>MVAPITTSGNKVLFGGQQGSIAGNSFFWSNTGWGGEKYYNAQTVAWLKSDWKSSLVRAAMGVDESGGYITDSYNKTRVTTVVDAAIANNMYVIIDWHSHHAEQYQSQAIAFFKEMATKYGNNNNVIYEIYNEPLQVSWSSVIKPYATAVIAEIRKIDPDNLIVVGTPTWSQDVDVAANDPITGYANIAYTLHFYAGTHGQSLRNKASTALSKGIPLFVTEWGSVNADGGGSVATAETNSWVSFMKTNNISNANWALNDKAEGASALVSGASANGGWTSSQLTASGTLAKSIISGWP[2x]

Here, we report a novel cellulase belonging to GH5 family, named as CelE1, retrieved from a sugarcane soil metagenomic library, which is a promising biocatalyst in biofuels production. CelE1 is 1284 bp long and encodes a polypeptide of 428 amino acid residues containing a putative N-terminal signal peptide followed by a glycoside hydrolase domain belonging to family 5 (GH5). Cellulases or endoglucanases (EC 3.2.1.4) catalyze the cleavage of random internal β-1,4-glycosidic bonds in cellulosic chains and can be found coupled to the cellulosome or generally secreted as independent enzymes. A new plant cell wall-degrading enzyme with ability to breakdown complex cellulose-based substrates was isolated and characterized from sugarcane soil metagenome. This enzyme was shown to be an endo-acting glucanase with high catalytic activity at a broad temperature range and under alkaline conditions that usually cause enzyme inactivation of classical acidic cellulases.

The structure of this novel cellulase 5 was determined by X-ray crystallography at 1.8 Å resolution. The crystals belonged to the monoclinic space group P21 with two molecules in the asymmetric unit, which could suggest a quaternary arrangement. However, analysis of crystalline contacts using the PDBePISA server did not indicate the presence of any stable protein–protein interface discarding the existence of CelE1 as a dimer in solution. The enzyme displays a canonical (β/α)8-barrel fold (also known as TIM-barrel) characteristic for members of GH5 family, which is composed by eight β-sheets surrounded by eight α-helices. The long loops connecting the C-terminal end of β-strands with the N-termini of the external layer of helices delineate the negatively charged catalytic cleft. By comparison with other cellulases the residues Glu152 and Glu240 were identified as the catalytic acidic residues, where Glu152 is the proton donor and Glu240 the nucleophile. These residues are separated by a distance of 6.1 Å, compatible for a retaining catalytic mechanism. Other important residues for catalysis are conserved including His117 and His212 and the aromatic gatekeepers Trp189 and Trp241. Despite the fully conserved catalytic cleft, some significant structural differences were found in the interfacial loops that vary in length and composition. Moreover, its crystal structure was determined at 1.8 Å resolution indicating that the 8-residue-long insertion in the β8-α8 loop might confer higher conformational stability in comparison to its psychrophilic orthologs.> GTAPKSRNLFERNPNKELKPGENSPRQTPIFDPTVHWLFTTCGASGPHGPTQAQCNNAYQNSNLSVEVGSEGPLKGIQIWKVPATDTYSISGYGAAGGKGGKNTMMRSHGVSVLGIFNLEKDDMLYILVGQQGEDACPSTNQLIQKVCIGENNVIEEEIRVNRSVHEWAGGGGGGGGATYVFKMKDGVPVPLIIAAGGGGRAYGAKTDTFHPERLENNSSVLGLNGNSGAAGGGGGW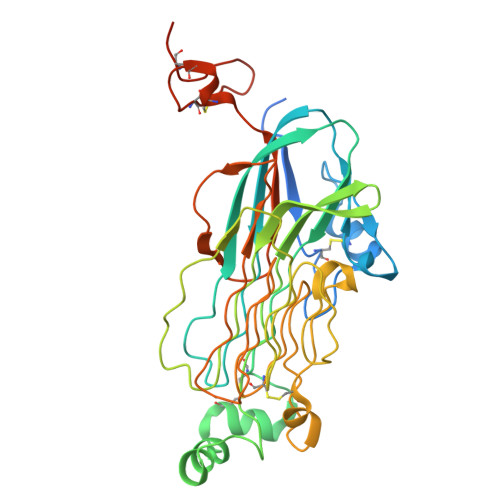NDNTSLLWAGKSLQEGATGGHSCPQAMKKWGWETRGGFGGGGGGCSSGGGGGGYIGGNAASNNDPEMDGEDGVSFISPLGILYTPALKVMEGHGEVNIKHYLNCSHCEVDECHMDPESHKVICFCDHGTVLAEDGVSCIVSP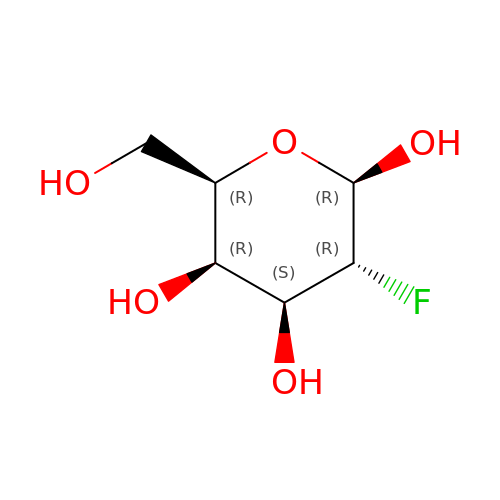2-deoxy-2-fluoro-beta-D-galactopyranose | C6 H11 F O5 | ZCXUVYAZINUVJD-VFUOTHLCSA-N>GMEVLDLVTGPDSVTEIEAFLNPRMGQPPTPESLTEGGQYYGWSRGINLATSDTEDSPENNTLPTWSMAKLQLPMLNEDLTCDTLQMWEAVSVKTEVVGSGSLLDVHGFNKPTDTVNTKGISTPVEGSQYHVFAVGGEPLDLQGLVTDARTKYKEEGVVTIKTITKKDMVNKDQVLNPISKAKLDKDGMYPVEIWHPDPAKNENTRYFGNYTGGTTTPPVLQFTNTLTTVLLDENGVGPLCKGEGLYLSCVDIMGWRVTRNYDVHHWRGLPRYFKITLRKRWVK[5x]

Murine Polyomavirus (MuPyV) is a double-stranded DNA virus that can induce tumors in newborn animals. Viral attachment is mediated by the major capsid protein, VP1, which forms pentameric capsomers that assemble into the T = 7d icosahedral capsid of the virus. Sialylated oligosaccharide receptors are engaged in a shallow groove on top of VP1 formed by loop structures on the protein surface, similar to other polyomaviruses. The differences among the three strains have been mapped to amino acid variations at two positions, 91 and 296, within the receptor-binding region of VP1.

The laboratory-derived RA strain shows limited spread and induces few tumors of strictly mesenchymal origin after a long latency period, while the naturally occurring PTA strain has disseminated infection and causes multiple tumors of epithelial and mesenchymal origin within a short time. MuPyV found in feral mice has the VP1 sequence of PTA, but the virus is controlled by an intact immune system. While RA bears a glycine residue at position 91, this residue is replaced with a glutamate in both PTA and LID. While the receptor interaction pocket of RA VP1 has been described, no structural information for the pathogenicity-defining amino acids at positions 91 and 296 in the pockets of PTA and LID has been available. PTA and LID both carry a glutamate at position 91, and this side chain is being held in a characteristic position with the carboxyl group facing away from the glycan receptor due to a salt bridge formed with K186, as previously predicted.>MPSKKNGRSGPQPHKRWVFTLNNPSEDERKKIRELPISLFDYFIVGEEGNEEGRTPHLQGFANFVKKQTFNKVKWYFGARCHIEKAKGTDQQNKEYCSKEGNLLMECGAPRSQGQRSDLSTAVSTLLESGSLVTVAEQHPVTFVRNFRGLAELLKVSGKMQKRDWKTNVHVIVGPPGCGKSKWAANFADPETTYWKPPRNKWWDGYHGEEVVVIDDFYGWLPWDDLLRLCDRYPLTVETKGGTVPFLARSILITSNQTPLEWYSSTAVPA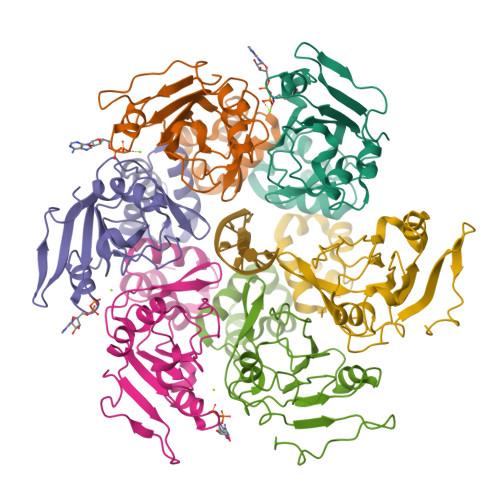VEALYRRITSLVFWKNATEQSTEEGGQFVTLSPPCPEFPYEINY[6x]(4-fluorophenoxy)acetic acid | C8 H7 F O3 | 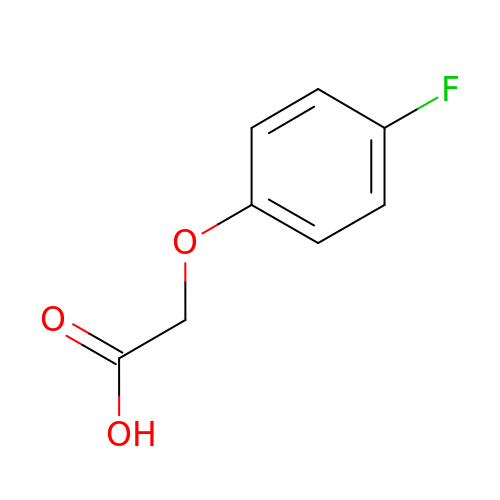ZBIULCVFFJJYTN-UHFFFAOYSA-N3,4-dimethoxy-N-({3-[(5-methyl-4,5,6,7-tetrahydro[1,3]thiazolo[5,4-c]pyridin-2-yl)carbamoyl]phenyl}methyl)benzamide | C24 H26 N4 O4 S 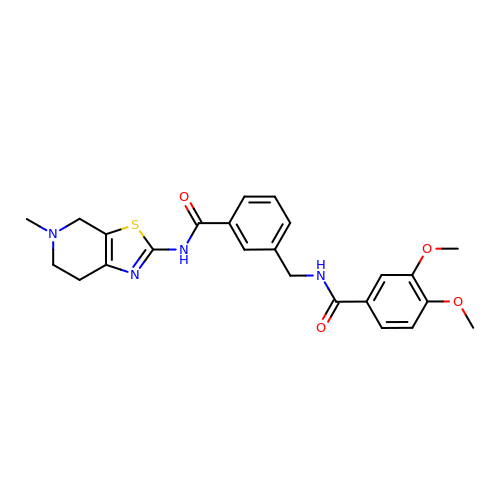| FDNORQUIWSIWKF-UHFFFAOYSA-N> MGSSHHHHHHSQDPMVAQQKNLEGYVGFANLPNQVYRK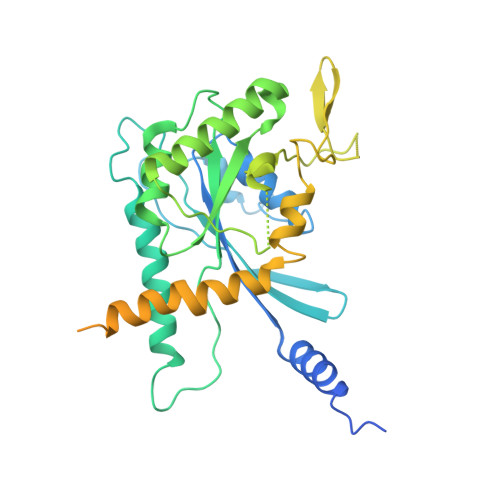SVKRGFEFTLMVVGESGLGKSTLINSLFLTDLYSPEYPGPSHRIKKTVQVEQSKVLIKEGGVQLLLTIVDTPGFGDAVDNSNCWQPVIDYIDSKFEDYLNAESRVNRRQMPDNRVQCCLYFIAPSGHGLKPLDIEFMKRLHEKVNIIPLIAKADTLTPEECQQFKKQIMKEIQEHKIKIYEFPETDDEEENKLVKKIKDRLPLAVVGSNTIIEVNGKRVRGRQYPWGVAEVENGEHCDFTILRNMLIRTHMQDLKDVTNNVHYENYRSRKLAAVTYNGVDNNKNKGQLTKSPLAQMEEERREHVAKMKKMEMEMEQVFEMKVKEKVQKLKDSEAELQRRHEQMKKNLEAQHKELEEKRRQFEDEKANWEAQQRILEQQNSSRTLEKNKKKGKIF>[12x]MAHHHHHHMKRLVPQFSKSSRNGVRHYSTLKQRGEKMDAELS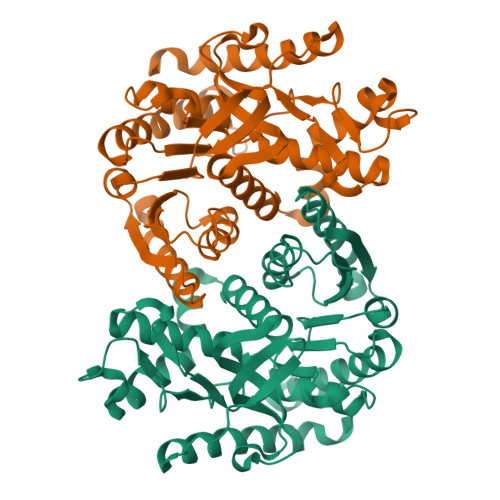ATRTPLERMLLGKQTKNDFANLNIKDPKTVAQWLNKSAREGPKYLTKDVDQLAPPVTITVSGACGQIANSLLFRIANGEMLGENQPVKLRLLERPEAMKALEGVKMELDDGAFPLLEEIYLTDSENDAFRGADYAILLGGKPRGPGMERADVMKDNAAIFKAQGEALNKQANGDVLVLIVANPANTNAMITSANAPDIPPENITAMTRLDHDRGLAQVAAKVGCNITDISRFAIWGNHSATQYPDLSFTTIKGQWGLNVINDEQWITNEFIPNVQQRGAAIIKARGKSSAASAADAAIKHMHDWVLGNSEWVSMAIPSRGQYGIPRGIWCSMPVQCFGAGKYGVIEGLPINSFSADRINASVKELIEEKKIVENLLPNPVYRLVEVDKVNIISKSYISENKQ> PEEIRPKEVYLDRKLLTLEDKELGSGNFGTVKKGYYQMKKVVKTVAVKILKNEANDPALKDELLAEANVMQQLDNPYIVRMIGICEAESWMLVMEMAELGPL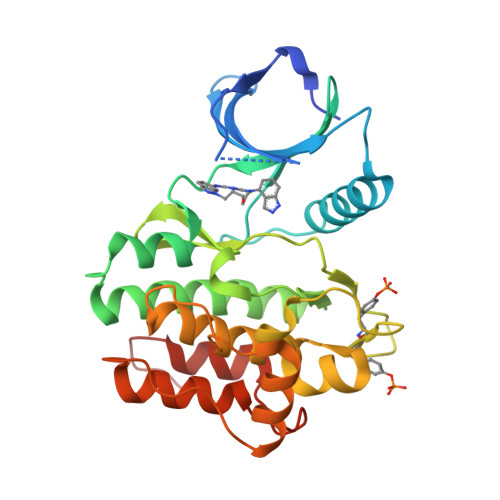NKYLQQNRHVKDKNIIELVHQVSMGMKYLEESNFVHRDLAARNVLLVTQHYAKISDFGLSKALRADENYYKAQTHGKWPVKWYAPECINYYKFSSKSDVWSFGVLMWEAFSYGQKPYRGMKGSEVTAMLEKGERMGCPAGCPREMYDLMNLCWTYDVENRPGFAAVELRLRNYYYDVVN>[2x]ARKCSLTGKWTNNLGSIMTIRAVNSRGEFTGTYLTAVADNPGNITLSPLLGIQHKRASQPTFGFTVHWNFSESTTVFTGQCFIDRNGKEVLKTMWLLRSSVNDISYDWKATL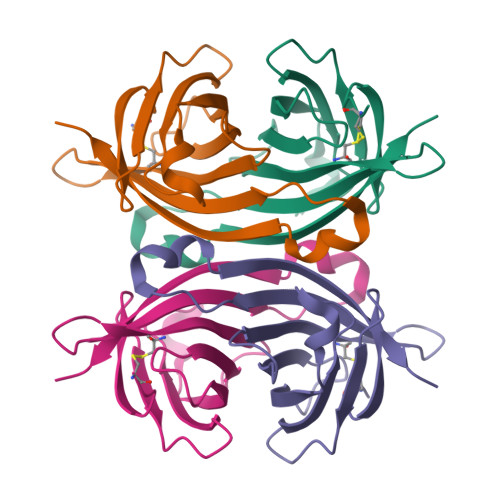VGYNNFTRLSTVEE>MADKELKFLVVDDFSTMRRIVRNLLKELGFNNVEEAEDGVDALNKLQAGGYGFVISDWNMPNMDGLELLKTIRADGAMSALPVLMVTVEAKKENIIAAAQAGASGYVVK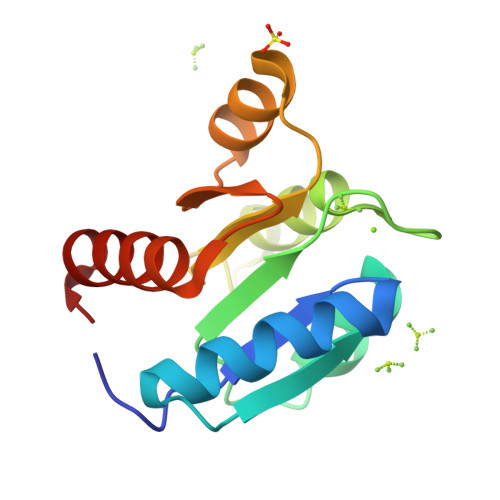PFTAATLEEKLNKIFEKLGM[2x]tridecanethial 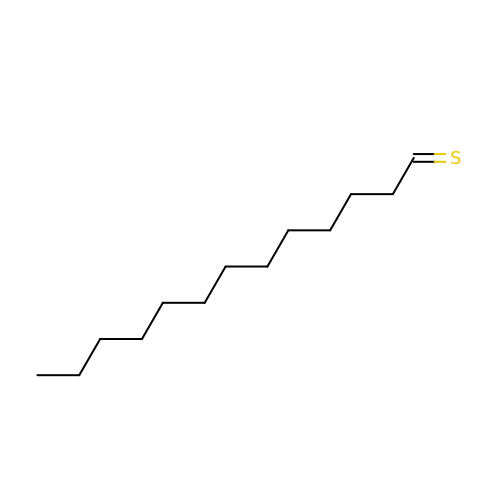| C13 H26 S | OPHBCQJSGYOCBI-UHFFFAOYSA-N> MTQELGNANFENFIGATEGFSEIAYQFTSHILTLGYAVMLAGLLYFILTIKNVDKKFQMSNILSAVVMVSAFLLLYAQAQNWTSSFTFNEEVGRY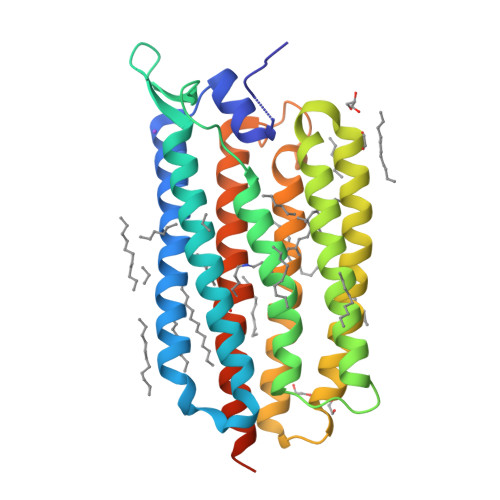FLDPSGDLFNNGYRYLNWLIDVPMLLFQILFVVSLTTSKFSSVRNQFWFSGAMMIITGFIGQFYEVSNLTAFLVWGAISSAFFFHILWVMKKVINEGKEGISPAGQKILSNIWILFLISWTLYPGAYLMPYLTGVDGFLYSEDGVMARQLVYTIADVSSKVIYGVLLGNLAITLSKNKELVEANSLEHHHHHH6-{[3-(dimethylamino)benzyl]amino}pyridine-3-carboxamide | C15 H18 N4 O | 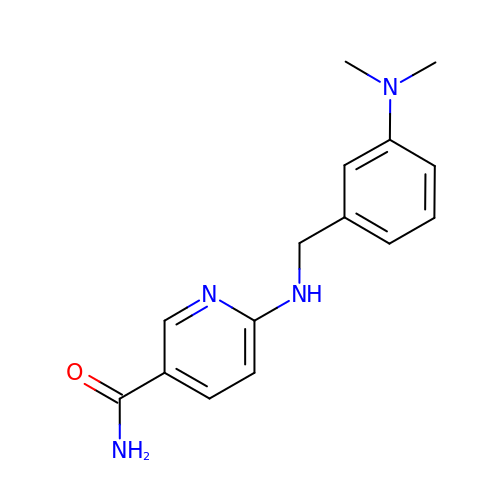RDIFHHLWNIKHIH-UHFFFAOYSA-N> MAEVSFGIELLPDDKPTKIAHLIKVAEDNGFEYAWICDHYNNYSYMGVLTLAAVITSKIKLGPGITNPYTRHPLITASNIATLDWISGGRAIIGMGPGDKATFDKMGLPFPCKIPIWNPEAEDEVGPATAIREVKEVIYQYLEGGPVEYEGKYVKTGTADVKARSIQGSDIPFYMGAQGPIMLKTAGEIANGVLVNASNPKDFEVAVPKIEEGAKEAGRSLDEIDVAAYTCFSIDKDEDKAIEATKIVVAFIVMGSPDVVLERHGIDTEKAEQIAEAIGKGDFGTAIGLVDEDMIEAFSIAGDPDTVVDKIEELLKAGVTQVVVGSPIGPDKEKAIELVGQEVIPHFK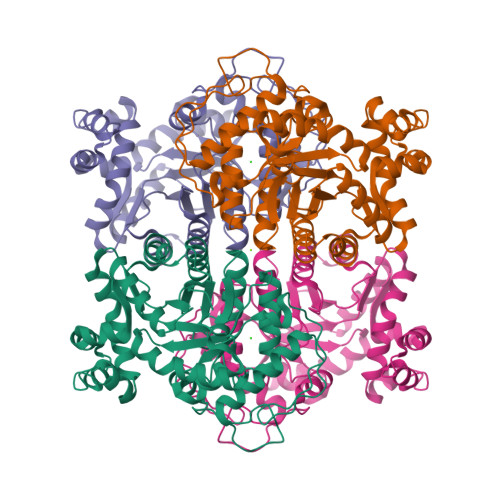E> GAMDPEFQQSKVAPSSAASRPVLSSRSDQSQKNEVFLDVVERLSVLIASNGSLLKVDVQGEIRLKSFLPSGSEMRIGLTEEFSVGKSELRGYGPGIRVDEVSFHSSVNLDEFESHRILRLQPPQGELTVMRYQLSDDLPSPLPFRLFPSVQWDRGSGRLQVYLKLRCDLLSKSQALNVRLHLPLPRGVVSLSQELSSPEQKAELAEGALRWDLPRVQGGSQLSGLFQMDVPGPPGPPSHGLSTSASPLGLGPASLSFELPRHTC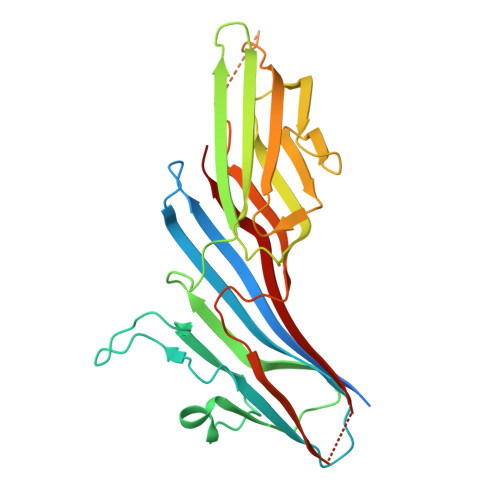SGLQVRFLRLAFRPSGNANPHKWVRHLSHSDAYVIRI THIAMPHENICOL | C12 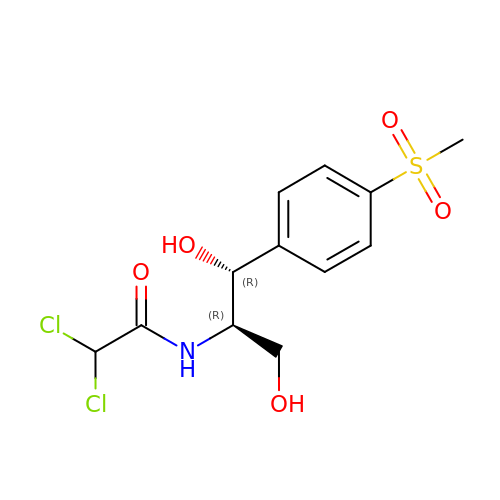H15 Cl2 N O5 S | OTVAEFIXJLOWRX-NXEZZACHSA-N>SWQTYVDEHLMCDIDGQGQQLAASAIVGHDGSVWAQSSSFPQFKPQEITGIMKDFEEPGHLAPTGLHLGGIKYMVIQGEAGAVIRGKKGSGGITIKKTGQALVFGIYEEPVTPGQCNMVVERLGDYLI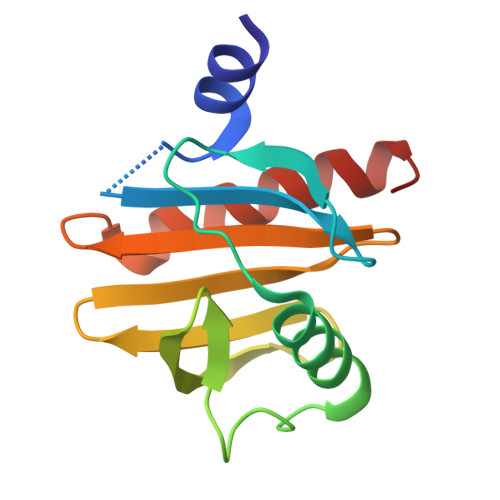DQGL[2x]>MWADIYHKLVEIYDIKAVKF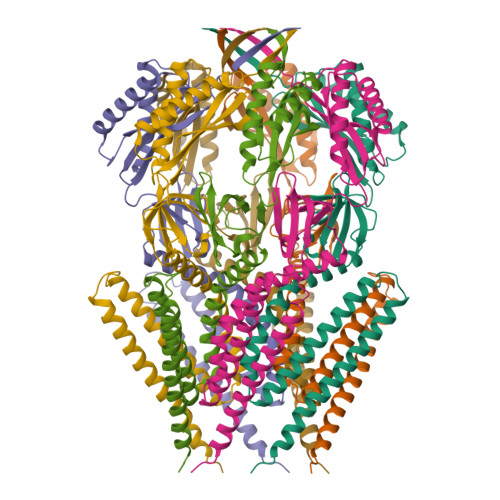LLDVLKILIIAFIGIKFADFLIYRFYKLYSKSKIQLPQRKIDTLTSLTKNAVRYIIYFLAGASILKLFNIDMTSLLAVAGIGSLAIGFGAQNLVKDMISGFFIIFEDQFSVGDYVTINGISGTVEEIGLRVTKIRGFSDGLHIIPNGEIKMVTNLTKDSMMAVVNIAFPIDEDVDKIIEGLQEICEEVKKSRDDLIEGPTVLGITDMQDSKLVIMVYAKTQPMQKWAVERDIRYRVKKMFDQKNISFPYPQMDVNFKRVKEDKAA[7x]> GPPGPKGDPGPKGDPGPPGARGQAGVLGFPGPPGPPGPKGDKGDPGGYX;> XGPPGPKGDPGPKGDPGPPGARGQAGVLGFPGPPGPPGPKGDKGDPGGYX;> XGPKGPPGDK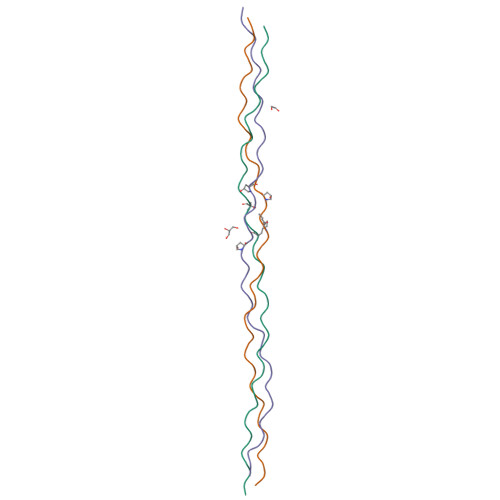GPPGDPGPPGARGEPGNIGFPGPPGPKGPKGDPGDPGGY>[5x]MSDIFNSPQNKASILTALMKSTTGDVEDVLIPKRFRPAKDPLDSPQAAAQFLKDNKYRILRPRAIPTMVELETDAALPRLRQMVEDGKLKDTVSVPEGTTAFYPKYYPFHKPDHDEVGTFGAPDITLLKQLTFFLLENDFPTGPETLRQVREAIATLQYGSGSYSGQLNRLLAMKGVATGRNPNKTPKTVGYTNEQLAKLLEQTLPINTPKHEDPDLRWAPSWLINYTGDLSTDKSYLPHVTIKSSAGLPYIGKTKGDTTAEALVLADSFIRDLGRAATSADPEAGVKKTITDFWYLSCGLLFPKGERYTQVDWDKKTRNIWSAPYPTHLLLSMVSTPVMNESKLNITNTQTPSLYGFSPFHGGMDRIMTIIRDSLDNDEDLVMIYADNIYILQDNTWYSIDLEKGEANCTPQHMQAMMYYLLTRGWTNEDGSPRYNPTWATFAMNVAPSMVVDSSCLLMNLQLKTYGQGSGNAFTFLNNH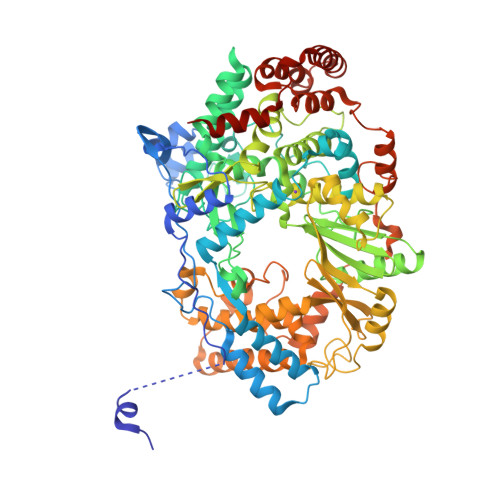LMSTIVVAEWVKAGKPNPMTKEFMDLEEKTGINFKIERELKNLRETIVEAVETAPQDGYLADGSDLPPIRPGKAVELDLLGWSAIYSRQMEMFVPVLENERLIASAAYPKGLENKALARKPGAEIAYQIVRYEAIRLVGGWNNPLLETAAKHMSLDKRKRLEVKGIDVTGFLDDWNNMSEFGGDLEGITLSEPLTNQTLVDINTPLDSFDPKARPQTPRSPKKTLDEVTTAITSGTYKDPKSAVWRLLDQRTKLRVSTLRDQALALKPASSSVDNWAEATEELAQQQQLLMKANNLLKSSLTETREALEKTGHHHHHH> KVLKISQTKYEEILKISKKYIFINQVDKSFHEAVDDLNQQDFIAVSGDGANMGRKCKMPFLVLSTDHQIYIFDIQVMQYHAFESGLKKILEGDSPRKIAHDCRKLSDCLYHKHNVKLKSVFDTQVGDLIITKNKKVTLPNKVKSLGECLTNYLGLQQNTIDEKLDIVQSTERPLSVKIKDSLARNIAFL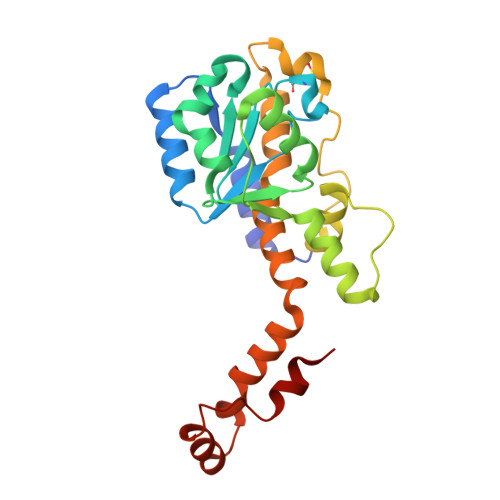HHLSEVINEEMQLPFYRGVECYIENIRSSDDFKAWELCGKLNQIPKEFRNAIDY The ferrous iron and 2-oxoglutarate (2OG)-dependent HIF prolyl hydroxylases (PHDs/EGLNs) catalyse trans-4-prolyl hydroxylations on HIFα subunits, thus promoting their binding to the von Hippel–Lindau protein (VHL), a targeting component of a ubiquitin E3 ligase, and signalling for HIFα degradation under normoxic conditions. The PHD-catalysed hydroxylations of HIF-1α/HIF-2α in higher animals occur in amino- and carboxy-terminal oxygen-dependent degradation domains (NODD and CODD). The three human PHDs exhibit different NODD/CODD selectivities, with PHD3 being substantially more selective for CODD than PHD1/2 (refs 16). Biophysical analyses employing crystallography and NMR reveal that the molecular basis of PHD isoform and variant selectivity involves enzyme–substrate interactions involving β2/β3 loop residues (that bind the LXXLAP motif) and helices α3 and α4, regions which display sequence variations between the PHD isoforms.

We obtained a PHD2.2OG.CODD structure using the strategy used for the PHD2.NOG.CODD complex, but did not obtain PHD2.NODD crystals using this procedure, possibly because NODD binds PHD2 less tightly, as indicated by a lower dissociation rate constant (kd) for CODD compared with NODD29. Notably, β2/β3 loop residues (Val241, Ser242, Lys244 and Ile251) interact with the ‘XX' residues of the LXXLAP motif, which differ in NODD and CODD (Glu560/Met561CODD; Thr398/Leu399NODD). In addition, CODD, but not NODD, interacts with α4 including via salt-bridging (Asp571CODD–Arg396PHD2). In the PHD2.CODD structure, Arg396PHD2 (α4) is positioned to salt bridge with Asp571CODD; analysis of the ODD structures leads to the prediction that the R396T and R396A substitutions disrupt their interaction with Asp571CODD, but will not directly have an impact on NODD binding. Consistent with the crystallographic results, large chemical shift perturbations manifested at the PHD2.CODD binding interface including in the β2/β3 loop region and α4; 15N relaxation and heteronuclear NOE measurements reveal the dynamic nature of these regions, particularly the β2/β3 loop. Comparison of the ODD complex structures and those without substrate reveals clear differences in NODD/CODD binding, especially in β2/β3 loop and C-terminal regions.

>GSHMASPNGQTKPLPALKLALEYIVPAMNKHGICVVDDFLGKETGQQIGDEVRALHDTGKFTDGQLVSQKSDSSKDIRGDKITWIEGKEPGCETIGLLMSSMDDLIRHCNGKLGSYKINGRTKAMVACYPGNGTGYVRHVDNPNGDGRCVTCIYYLNKDWDAKVSGGILRIFPEGKAQFADIEPKFDRLLFFWSDRRNPHEVQPAYATRYAITVWYFDADERAAAKVKYLTGEKGVRVELNKPSDSVGKDVF[2x];>[2x]DLDLEMLAPYIPMDDDFQL> EPVVDTPHPGEALYEAQCASCHGKDGKGGLAGGELLGCDVCGDFSLLALRIEQTMPLGNPEQCDTQCSSQIAGYMLENFAGLPPTLEHHHHHH

We therefore set out to characterize two previously unstudied proteins from the shipworm symbiont Teredinibacter turnerae that were initially identified by the presence of carbohydrate binding domains appended to uncharacterized domains with probable redox functions. One of these was TERTU_3803, which contained both a CBM10 and a CBM2 domain attached to a range of distinct modules (via flexible linkers) that did not bare any sequence similarity with catalytic domains typically found within carbohydrate-active enzymes. Using a ‘module walking’ approach, we searched for other genes coding for these X-domains. This led to the identification of TERTU_2913, which lacks CBMs but contains predicted X122, X183 and X132 domains. Taken together, these sequence analyses suggested that TERTU_3803 and TERTU_2913 could have a role to play in cellulose metabolism, and furthermore that role is likely to be a redox one given the presence of cytochrome domains within their linear amino acid sequences.

TtX183A, TtX183B and TtX183C, which all derive from TERTU_2913, were expressed and purified from the E. coli periplasm following co-expression with the cytochrome maturation machinery encoded on the pEC86 plasmid. All three proteins underwent crystal trials but only TtX183A and TtX183B formed diffracting crystals. The structure for TtX183A was determined via single-wavelength anomalous dispersion from the anomalous signal generated by the haem iron to a resolution of 1.4 Å. The resulting model was subsequently used to determine the structure of TtX183B via molecular replacement to 1.8 Å resolution. The polypeptide chain in each of TtX183A and TtX183B fold around the haem to produce a tertiary structure dominated by α-helices, as expected for small c-type cytochromes [Fig. 2(a)]. To examine the structural similarities within our TtX183 domain structures, we compared TtX183A with TtX183B and found that the structures superposed with one another with an r.m.s.d. of 1.12 Å over 59 Cα positions. In the structures of TtX183A and TtX183B, the haem propionate groups are highly solvent exposed where in CjX183 a loop was found to interact with these groups. This is likely to provide an easier exit route for electrons when O2 is present, explaining the apparent lack of stability of the reduced state for the TtX183s compared with CjX183.> MKQDASRNAAYTVDCEDYVHVVEFNPFENGDSGNLIAYGGNNYVVIGTCTFQEEEADVEGIQYKTLRTFHHGVRVDGIAWSPETRLDSLPPVIKFCTSAADMKIRLFTSDLQDKNEYKVLEGHTDFINGLVFDPKEGQEIASVSDDHTCRIWNLEGVQTAHFVLHSPGMSVCWHPEETFKLMVAEKNGTIRFYDLLAQQAILSLESEQV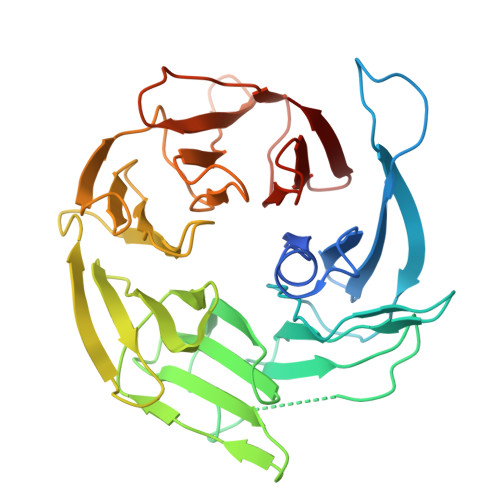PLMSAHWCLKNTFKVGAVAGNDWLIWDITRSSYPQNKRPVHMDRACLFRWSTISENLFATTGYPGKMASQFQIHHLGHPQPILMGSVAVGSGLSWHRTLPLCVIGGDHKLLFWVTEV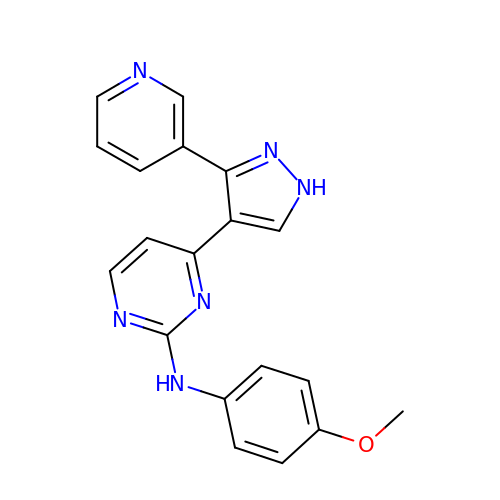N-(4-methoxyphenyl)-4-[3-(pyridin-3-yl)-1H-pyrazol-4-yl]pyrimidin-2-amine | C19 H16 N6 O | ANTWQGSNXAZMBT-UHFFFAOYSA-N>GSWSVKELEDKNEELLSEIAHLKNEVARLKKLLQRCLAANQELRDAMRQSNQILRERAEELLHFQASQREEKEFLMSKFQEARKLVERLGLEKLELEDKNEELLSEIAHLKNEVARLKKLVGER[2x]

Inhibition of the protein-protein interaction between NEMO and IKKβ represents an attractive alternative strategy due to the crucial role of NEMO and its selective involvement in the canonical NF-κB pathway. We have previously reported the design and characterization of a coiled-coil stabilized NEMO construct encompassing the IKKβ-binding region fused to two ideal dimeric coiled-coil adaptors, at the N and C-terminus. Here we report the structure of the unliganded N-terminal domain of NEMO, utilizing the coiled-coil stabilized NEMO construct modified by four additional point mutations, designed to improve solution behavior and crystal packing. The crystal structure reveals that NEMO folds in an irregular dimeric coiled coil in the absence of IKKβ, with discontinuities in the heptad repeats causing an underwinding of the supercoil in the ligand binding region.

The mutation I65M was introduced to provide an additional site for selenomethionine labeling, to aid in phase determination (NEMO-I65M). Ile65 was chosen for its expected buried position within the coiled coil, providing a more rigid methionine than that of the natural sequence Met94. The SeMet labeled I65M mutant was prepared to facilitate the phasing of the EEAA structure, but displayed weak anomalous signal, and the structures were instead solved by molecular replacement. The I65M mutation affects the opening of the hot-dog bun increasing the interhelical spacing of the three heptad repeats starting at residues 65, 72 and 79 to the values observed in the IKKβ-bound structure. The longer side chain of Met65 extends deep in the interhelical cleft and the structure accommodates it by increasing the interhelical spacing by 1.4 Å and rotating the second Met65′ away from the center of the bun. This increased spacing seems to trigger the opening of the bun in the following heptads, till the end of the stutter “heptad”. The open region encompasses ligand binding pockets I and II. After residue 82, and approximately at the start of pocket III, the I65M structure closes back to resemble the apo structure, confirming the role of IKKβ in maintaining an open pocket III. The conformation of pocket III is instead almost identical in the I65M mutant and NEMO-EEAA structure, both in interhelical spacing and in side chain conformations, with an RMSD = 0.372 Å over all backbone atoms within residues 89–104. The data suggest that NEMO-I65M unfolds more easily and more completely than the other two constructs, due to the prevention of a compact packing of the dimer at the beginning of the discontinuous region, caused by Met65, and destabilization of the packed regions of the coiled coil.>ISEFGSSMGLAELRELIEPEETDLRALAGREIAIDAFNALYQFLTTIMKDGRPLMDSRGRITSHLNGLLYRTVNLVEEGIKPVYVFDGEPPDLKRETLERRRERKEEAMEKLRRAKTKEEREKYARQVARLDESLVE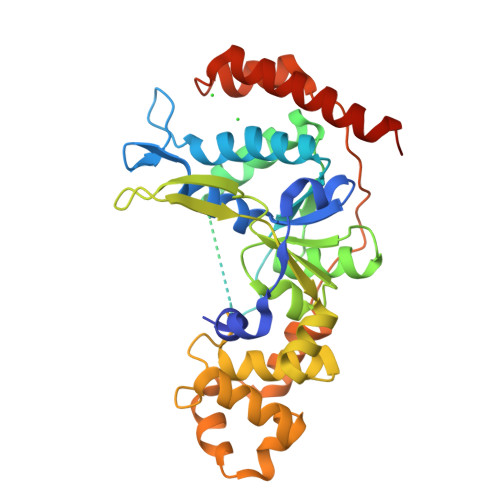DAKRLLDLMGIPWVQAPSEGEAQCAYMARCGDVWATGSQDYDSLLFGSPRLVRNITIVGKRKHPHTGEIIEVKPEIMRLEDVLDQLGLESREQLVDLAILLGTDYNPDGVPGIGPKRALQLIRKYGSLDELKDTDIWPKIERHLPVEPEKLRRLFLEPEVTDDYELDWDEPDEEGLVEFLVEERDFSEDRVRRAVERLKEALQELRKGGRQETLDAFF[2x]5-[(2,4-dichlorobenzyl)sulfanyl]-4H-1,2,4-triazol-3-amine | C9 H8 Cl2 N4 S | 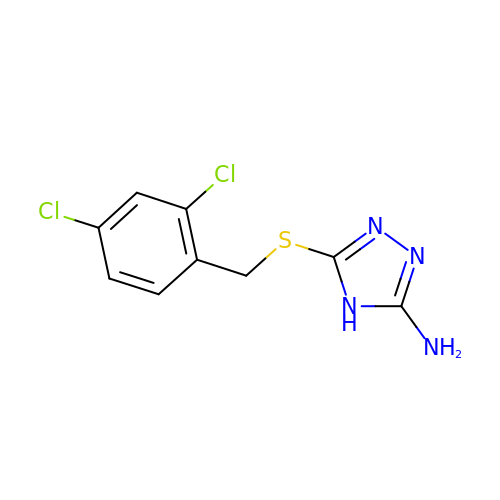ZOVIHJUPKVOGKF-UHFFFAOYSA-N>[4x]MAYVPAPGYQPTYNPTLPYYQPIPGGLNVGMSVYIQGVASEHMKR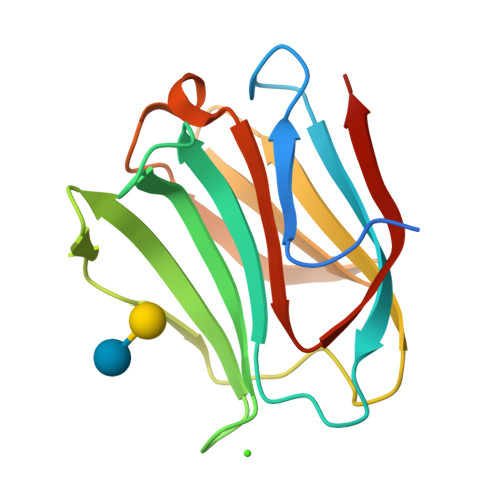FFVNFVVGQDPGSDVAFHFNPRFDGWDKVVFNTLQGGKWGSEERKRSMPFKKGAAFELVFIVLAEHYKVVVNGNPFYEYGHRLPLQMVTHLQVDGDLQLQSINFIGGQPL> CIKCDQFVTDALKTFENTYLNDHLPHDIHKNVMRMVNHEVSSFGVVTSAEDSYLGAVDENTLEQATWSFLKDLKRITDSDLKGELFIKELLWMLRHQKDIFNNLARQFQKEVLCPNKCGVMSQTLIWCLKCEKQ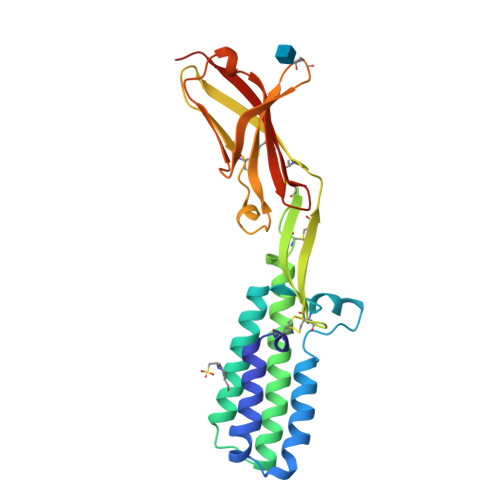LHICRKSLDCGERHIEVHRSEDLVLDCLLSWHRASKGLTDYSFYRVWENSSETLIAKGKEPYLTKSMVGPEDAGNYRCVLDTINQGHATVIRYDVTVLPPKH>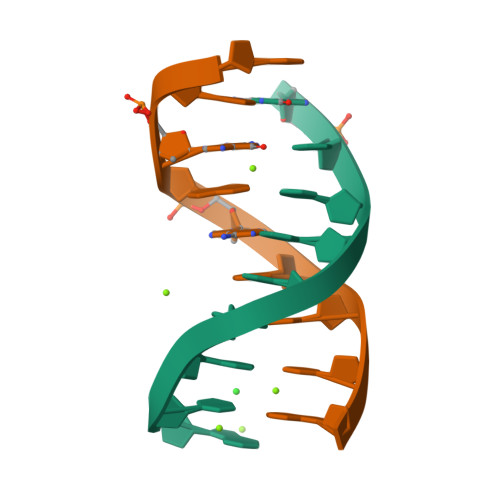[2x]GCGAATTCG>GTNTNLQTFELPTEVTGCAADISLGRALIQAWQKDGIFQIKTDSEQDRKTQEAMAASKQFCKEPLTFKSSCVSDLTYSGYVASGEEVTAGKPDFPEIFTVCKDLSVGDQRVKAGWPCHGPVPWPNNTYQKSMKTFMEELGLAGERLLKLTALGFELPINTFTDLTRDGWHHMRVLRFPPQTSTLSRGIGAHTDYGLLVIAAQDDVGGLYIRPPVEGEKRNRNWLPGESSAGMFEHDEPWTFVTPTPGVWTVFPGDILQFMTGGQLLSTPHKVK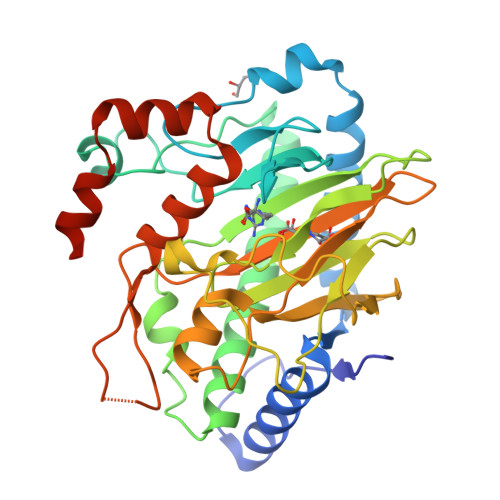LNTRERFACAYFHEPNFEASAYPLFEPSANERIHYGEHFTNMFMRCYPDRITTQRINKENRLAHLEDLKKYSDTRATGS[4x]>PFTYSIEATRNLATTERCIQDIRNAPVRNRSTQFQLAQQNMLAYTFGEVIPGFASAGINGMDYRDVIGRPVENAVTEGTHFFRDDFRVDSNAKAKVAGDIFEIVSSAVMWNCAARWNSLMVGEGWRSQPRYSRPTLSPSPRRQVAVLNLPRSFDWVSLLVPESQEVIEEFRAGLRKDGLGLPTSTPDLAVVVLPEEFQNDEMWREEIAGLTRPNQILLSGAYQRLQGRVQPGEISLAVAFKRSLRSDRLYQPLYEANVMQLLLEGKLGAPKVEFEVHTLAPEGTNAFVTYEAASLYGL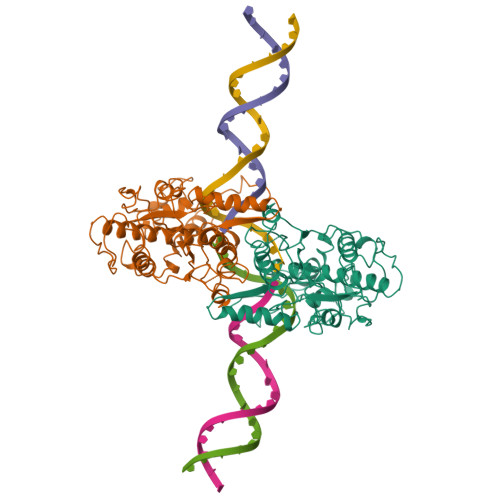AEGRSAVHRAIRELYVPPTAADLARRFFAFLNERMELVN[2x]> MSIVSRQNANTYSAEGRLYQVEYAMQAMNLGTSSIGIKTKDYVLLASEKKIISKLQNPSSVKKHYRVYDHIALGFSGISADVKTIVDKSRNFAINHEYLYDENCKVERLLEHLADLSLNFDKKEADEKIFSRPFGASLLIIGYDTEPRLFSLDPSGS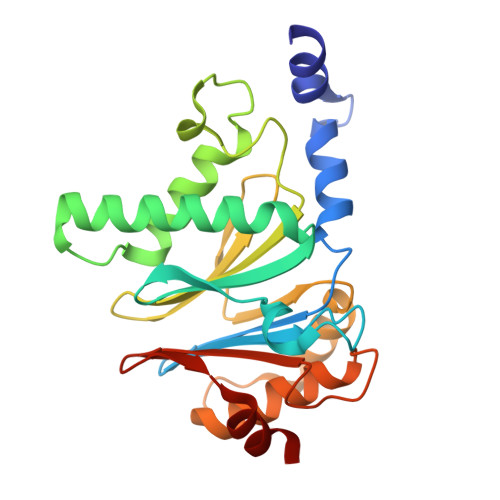YLEYHAKAIGSGSEVIENMLEQEFDPNVDINSGLKNILNMLSKVMKDKINNFNVEITAITKNECKILTPEEIEQFLE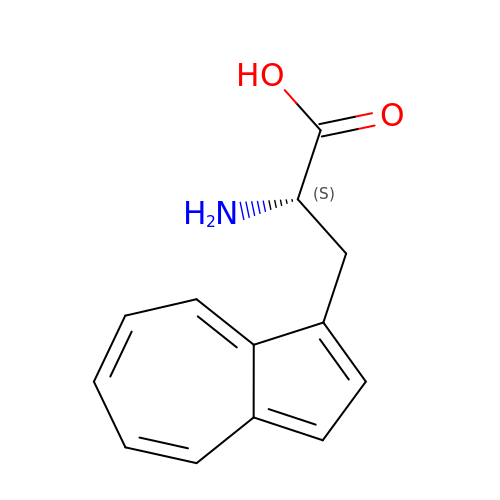beta-(1-azulenyl)-L-alanine | C13 H13 N O2 | OFJOITXZODXNIG-LBPRGKRZSA-N> GPGGEMQKIVFKIPMVDDKSRTKAMSLVASTVGVHSVAIAGDLRDQVVVVGDGIDSINLVSALRKKVGPAMFLEVSQV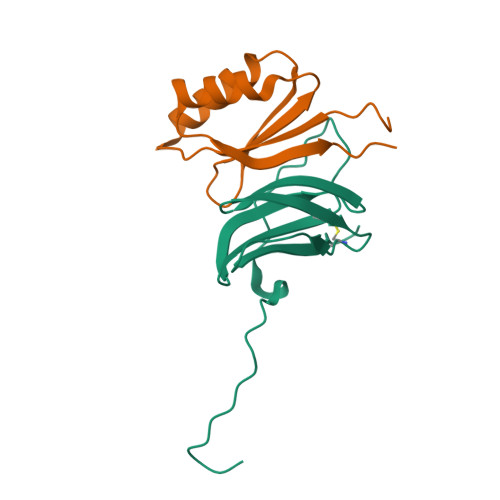KED;> METGNKYIEKRAIDLSRERDPNFFDNPGIPVPECFWFMFKNNVRQDAGTCYSSWKMDMKVGPNWVHIKSDDNCNLSGDFPPGWIVLGKKRPGF> RAPDSVDYRKKGYVTPVKNQGQCGSCWAFSSVGALEGQLKKKTGKLLNLSPQNLVDCVSENDGCGGGYMTNAFQYVQKNRGIDSEDAYPYVGQEESCMYNPTGKAAKCRGYREIPEGNEKALKRAVARVGPVSVAIDAS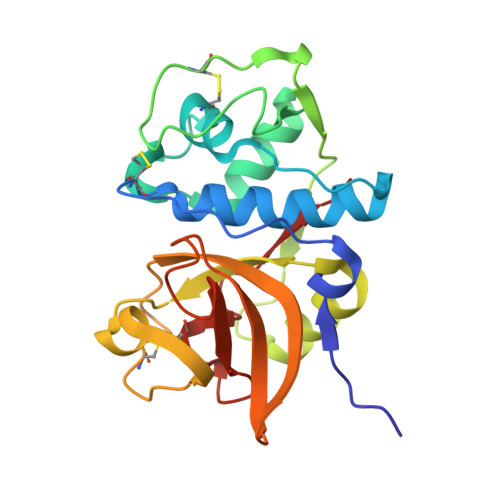LTSFQFYSKGVYYDESCNSDNLNHAVLAVGYGIQKGNKHWIIKNSWGENWGNKGYILMARNKNNACGIANLASFPKM> MAPVQLDNHQLIPPGGGGGSSGGGGSSSGSASAPAPPPPAAAVAAAAAAAASPGYRLSTLIEFLLHRAYSELMVLTDLLPRKSDVERKIEIVQFASRTRQLFVRLLALVKWANDAGKVEKCAMISSFLDQQAILFVDTADRLASLARDALVHARLPSFAIPYAIDVLTTGSYPRLPTCIRDKIIPPDPITKIEKQATLHQLNQILRHRLVTTDLPPQLANLTVANGRVKFRVEGEFEATLTVMGDDPEVPWRLLKLEILVEDKETGDGRALVHSMQIDFIHQLVQSRLFADEKPLQDMYNCLHCFCLSLQLEVLHSQTLMLIRERWGDLVQVERYHAGKSLSLSVWNQQVLGRKTGTASVHKVTIKIDENDVSKPLQIFHDPPLPASDSKLVERAMKIDHLSIEKLLIDSVHARAHQRLQELKAILRSFNANESSSIETALPALIVPILEPCGNSECLHIFVDLHSGMFQLMLYGLDPATLEDMEKSLNDDMKRIIPWIQQLKFWLGQQRCKQSIKHLPTITTETLQLANYSTHPIGSLSKNKLFIKLTRLPQYYIVVEMLEVPNKPTQLSYNYYFMSVSTADREDSPVMALLLQQFKDNIQDLMSYTKTGKQTRTGTKHKLSDDPCPIDSKKAKRSGEMCAFNKVLAHFVAMCDTNMPFVGLRLELSNLEIPHQGVQVEGDGFNHAIRLLKIPPCKGISEETQKALDRSLLDCTFRLQGRNNRTWVAELVFANCPLNGTSTREQGPSRHVYLTYENLLSEPVGGRKVVEMFLNDWSSIARLYECVLEFARSLPEIPAHLNIFSEVRVYNYRKLILCYGTTKGSSISIQWNSIHQKFHIALGTVGPNSGCSNCHNTILHQLQEMFNKTPNVVQLLQVLFDTQAPLNAINKLPTVPMLGLTQRTNTAYQCFSILPQSSTHIRLAFRNMYCIDIYCRSRGVVAIRDGAYSLFDNSKLVEGFYPAPGLKTFLNMFVDSNQDARRRSVNEDDNPPSPIGGDMMDSLISQLQPPQQQPFPKQPGTSGAYPLTSPPTSYHSTVNQSPSMMHTQSPGNLHAASSPSGALRAPSPASFVPTPPPSSHGISIGPGASFAS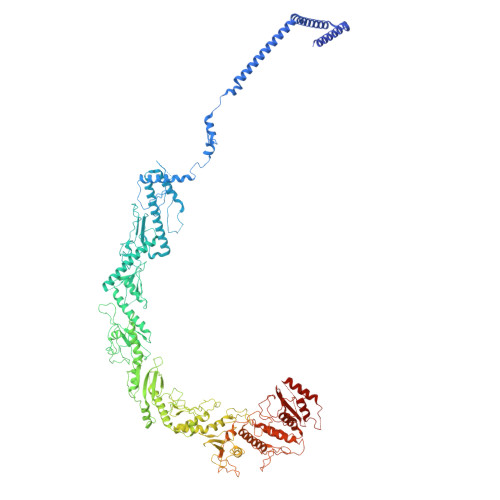PHGTLDPSSPYTMVSPSGRAGNWPGSPQVSGPSPATRLPGMSPANPSLHSPVPDVSHSPRAGTSSQTMPTNMPPPRKLPQRSWAASIPTILTHSALNILLLPSPTPGLVPGLAGSYLCSPLERFLGSVIMRRHLQRIIQQETLQLINSNEPGVIMFKTDALKCRVALSPKTNQTLQLKVTPENAGQWKPDELQVLEKFFETRVAGPPFKANTLIAFTKLLGAPTHILRDCVHIMKLELFPDQATQLKWNVQFCLTIPPSAPPIAPPGTPAVVLKSKMLFFLQLTQKTSVPPQEPVSIIVPIIYDMASGTTQQADIPRQQNSSVAAPMMVSNILKRFAEMNPPRQGECTIFAAVRDLMANLTLPPGGRP> GYDFVIDEITYNFTKEHGTVEVSGLREFLNLEPGDRNSSLPLVVNIPPVVTYKDNKYDVVSIGYAAFQGCRKVTEIKIPSTVREIGEFAFENCSKLEIINIPDSVKMIGRCTFSGCYALKSILLPLMLKSIGVEAFKGCDFKEITIPEGVTVIGDEAFATCESLEYVSLPDSMETLHNGLFSGCGKLKSIKLPRNLKIIRDYCFAECILLENMEFPNSL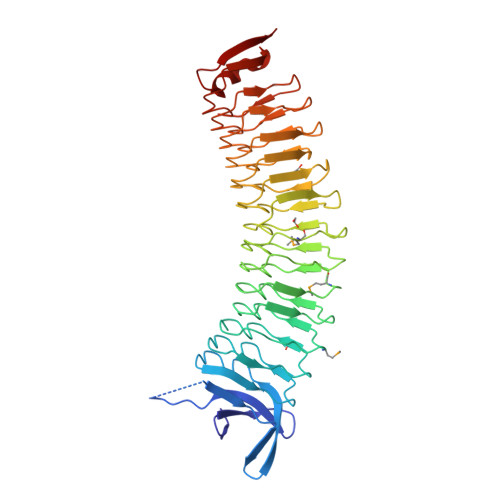YYLGDFALSKTGVKNIIIPDSFTELGKSVFYGCTDLESISIQNNKLRIGGSLFYNCSGLKKVIYGSVIVPEKTFYGCSSLTEVKLLDSVKFIGEEAFESCTSLVSIDLPYLVEEIGKRSFRGCTSLSNINFPLSLRKIGANAFQGCINLKKVELPKRLEQYRYDFEDTTKFKWIK> SMGECSQKGPVPFSHCLPTEKLQRCEKIGEGVFGEVFQTIADHTPVAIKIIAIEGPDLVNGSHQKTFEEILPEIIISKELSLLSGEVCNRTEGFIGLNSVHCVQGSYPPLLLKAWDHYNSTKGSANDRPDFFKDDQLFIVLEFEFGGIDLEQMRTKLSSLATAKSILHQLTASLAVAEASLRFEHRDLHWGNVLLKKTSLKKLHYTL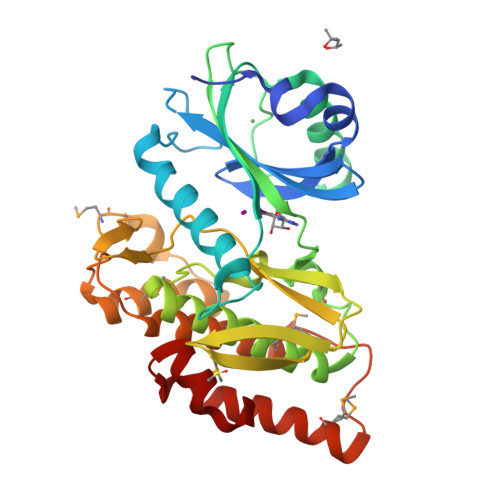NGKSSTIPSCGLQVSIIDYTLSRLERDGIVVFCDVSMDEDLFTGDGDYQFDIYRLMKKENNNRWGEYHPYSNVLWLHYLTDKMLKQMTFKTKCNTPAMKQIKRKIQEFHRTMLNFSSATDLLCQHSLFK>[8x]MAALTKVKLCQLDDLMPFIGATVLIEGE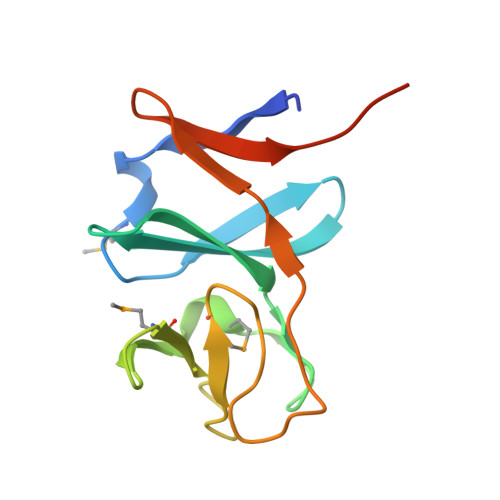RVALFYIPDSGVYAVQDWDPIGKAYVMSRGIVGDINGEMCVASPLYKQHFSLKSGQCLEDEAHCLKTWRVTVDDNQVCYLAKELEHHHHHH> MGNETVVVAETAGSIKVAVVVCLLRGQNVLLGRRRSSLGDSTFSLPSGHLEFGESFEECAARELKEETDLDIGKIELLTVTNNLFLDEAKPSQYVAVFMRAVLADPRQ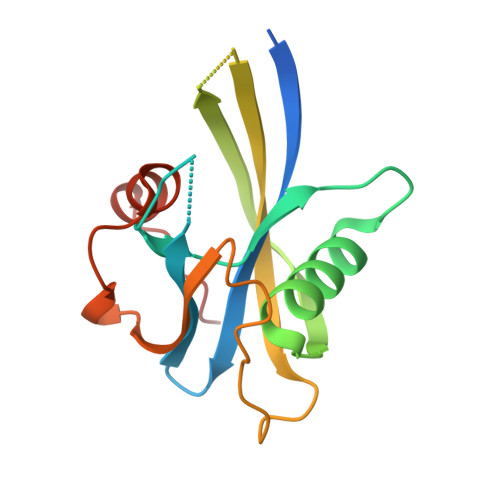EPQNIEPEFCDGWGWYEWDNLPKPLFWPLDNVVQDGFNPFPT Carbazole 1,9a-dioxygenase (CARDO), a RO member consists of catalytic terminal oxygenase (CARDO-O), ferredoxin (CARDO-F), and ferredoxin reductase. The mononuclear iron site activates dioxygen for reaction with the substrate, and the Rieske cluster transfers electrons to the mononuclear iron site during the catalytic cycle. In the present study, we determined the crystal structures of the reduced CAR-bound Oxy:Fd complex (Oxy: Fdred-CAR), oxygen-bound Oxy:Fd complex (Oxy: FdO2), and both CAR- and oxygen-bound Oxy:Fd complex (Oxy: FdCAR-O2) at 1.95, 1.85, and 2.0 Å resolution, respectively. All Oxy:Fd structures solved consist of one molecule of Oxy (comprising three subunits: chains A, B, and C) and three molecules of Fd (chains D, E, and F), and the asymmetric unit of the crystal contains one Oxy:Fd structure.

Oxy: Fdred-CAR provided the same observations as those of Oxy: FdCAR (2’), which were a clear density for a flat aromatic compound in the active site and the CAR-binding-dependent movement of amino acid residues Leu202–Thr214 and Asp229–Val238 toward the entrance of the substrate-binding pocket in chains B and C (data not shown). The electron density maps of CAR were only found in chains B and C, because the symmetry-related structure partially filled the entrance of the substrate-binding pocket in chain A. The active site of Oxy: Fdred-CAR showed a six-coordinate, distorted octahedral geometry with two water ligands, while that of Oxy: FdCAR (2’) could be described as a distorted tetragonal geometry with one water ligand. Notably, the nonheme iron and its ligand residue, Asp333, moved away from CAR by approximately 0.5 and 0.4 Å, respectively, in Oxy: Fdred-CAR. In chains B and C of Oxy: Fdred-CAR, the average bond lengths between mononuclear iron–Asp333OD1 and mononuclear iron–Asp333OD2 changed from 2.0 Å to 1.9 Å and from 2.6 Å to 2.2 Å, respectively, which made the coordination of the carboxylate residue to nonheme iron clearly bidentate. The slight movement of Phe67 in Oxy: Fdred-CAR was common in Oxy: Fdred, in which the single-crystal microspectrophotometer clearly confirmed the reduced status of the Rieske cluster. This suggests that this slight movement of Phe67 may be specific for reduction of the Rieske cluster. In the case of CARDO-O, reduction upon substrate binding triggered displacement of the nonheme iron and residues including Asp333 away from the substrate, which increased the accessible surface at the mononuclear iron, opened room for dioxygen binding, and allowed binding of an exogenous sixth water ligand. In other words, movement of the nonheme iron away from the substrate when the Rieske cluster is reduced might act as a physical mechanism of gating oxygen reactivity.

>[3x]MANVDEAILKRVKGWAPYVDAKLGFRNHWYPVMFSKEINEGEPKTLKLLGENLLVNRIDGKLYCLKDRCLHRGVQLSVKVECKTKSTITCWYHAWTYRWEDGVLCDILTNPTSAQIGRQKLKTYPVQEAKGCVFIYLGDGDPPPLARDTPPNFLDDDMEILGKNQIIKSNWRLAVENGFDPSHIYIHKDSILVKDNDLALPLGFAPGGDRKQQTRVVDDDVVGRKGVYDLIGEHGVPVFEGTIGGEVVREGAYGEKIVANDISIWLPGVLKVNPFPNPDMMQFEWYVPIDENTHYYFQTLGKPCANDEERKKYEQEFESKWKPMALEGFNNDDIWAREAMVDFYADDKGWVNEILFESDEAIVAWRKLASEHNQGIQTQAHVSGLEHHHHHH;>MNQIWLKVCAASDMQPGTIRRVNRVGAAPLAVYRVGDQFYATEDTCTHGIASLSEGTLDGDVIECPFHGGAFNVCTGMPASSPCTVPLGVFEVEVKEGEVYVAGEKKLEHHHHHH[3x]Monoamine neurotransmitters such as serotonin and dopamine are loaded by vesicular monoamine transporter 2 (VMAT2) into synaptic vesicles for storage and subsequent release in neurons. VMAT2 inhibitors reserpine and tetrabenazine are used to treat hypertension, movement disorders associated with Huntington’s Disease and Tardive Dyskinesia. Here we present cryo-EM structures of human apo VMAT2 in addition to states bound to serotonin, tetrabenazine, and reserpine. These structures collectively capture three states, namely the lumen-facing, occluded, and cytosol-facing conformations.

To capture the cytosol-facing state which was previously proposed to favor RES binding, we used the Y422C mutation (VMAT2YC) which was presumed to weaken the cytosolic gate. We then incubated VMAT2YC with 1 mM RES and determined a 3.7 Å structure (VMAT2YCR) at a cytosol-facing state. Compared with the lumen-facing VMAT2A state, the N- and C-domain of cytosol-facing VMAT2YCR structure undergo a typical rocker-switch movement, similar to other MFS transporters. An elongated density of ~20 Å was observed in the translocation funnel of VMAT2YCR map. This density matches the shape of the multi-ring RES. The RES trimethyoxylbenzoyl group faces the cytosolic space and is positioned nearly perpendicularly to its three adjacent rings in the middle. On the opposite side, the indole group is also perpendicular to the middle rings and is inserted snugly in the central cavity of VMAT2 transport passage. This indole group assumes a similar position of 5-HT, explaining its competitive nature. The tertiary amine on the middle tandem rings established hydrogen bond and salt bridge with Asn305 and Asp399, respectively, as well as a cation–π interaction with Tyr341. At the cytosolic vestibule, the trimethyoxylbenzoyl group brings in the cytosolic halves of the N- and C-domain by engaging with Leu225, Leu228, Met403, Ala425 and Phe429.

> MALSELALVRWLQESRRSRKLILFIVFLALLLDNMLLTVVVPIIPSYLYSIKHEKNATEIQTARPVHTASISDSFQSIFSYYDNSTMVTGNATRDLTLHQTATQHMVTNASAVPSDCPSEDKDLLNENVQVGLLFASKATVQLITNPFIGLLTNRIGYPIPIFAGFCIMFVSTIMFAFSSSYAFLLIARSLQGIGSSCSSVAGMGMLASVYTDDEERGNVMGIALGGLAMGVLVGPPFGSVLYEFVGKTAPFLVLAALVLLDGAIQLFVLQPSRVQPESQKGTPLTTLLKDPYILIAAGSICFANMGIAMLEPALPIWMMETMCSRKWQLGVAFLPASISYLIGTNIFGILAHKMGRWLCALLGMIIVGVSILCIPFAKNIYGLIAPNFGVGFAIGMVDSSMMPIMGYLVDLRHVSVYGSVCAIADVAFCMGYAIGPSAGGAIAKAIGFPWLMTIIGIIDILFAPLCFFLRSPPSRLEEELRRRTEGGSSDLEVLFQ> PTAIAICLYYKLGETPLPLVIETGKDAKALQIIKLAELYDIPVIEDIPLARSLYKNIHKGQYITEDFFEPVAQLIRIAIDL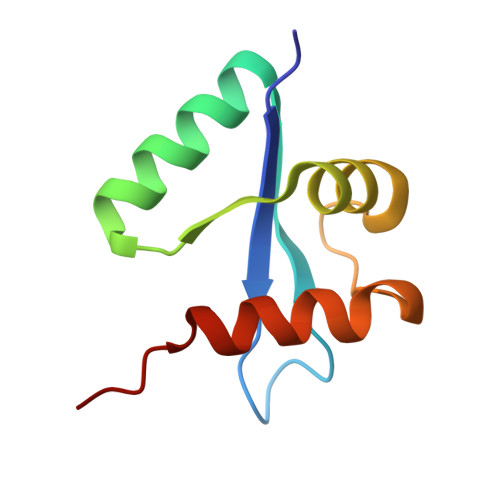DY The protein TON_0340 (268 amino acids) was identified in a transcriptome study aimed at identifying genes whose expression is enhanced when this organism was grown with CO as the sole carbon and energy source. The biological function of TON_0340 is unknown, and a BLAST database search shows that TON_0340 belongs to the DUF4392 superfamily (after domain of unknown function), the members of which are found in all three domains of life. To gain insights into the biochemical function of TON_0340 and its homologues, we determined the crystal structures of TON_0340 in four different forms; the apo form without a bound metal ion and the Mn2+-, Mg2+- or Ca2+-bound form, revealing that the protein has a highly conserved bi-metal binding pocket. Our analyses strongly support that TON_0340 is a novel Mn2+-dependent phosphatase.

The Ca2+-bound TON_0340 structure was determined by growing the crystals in the presence of CaCl2. Unexpectedly, only one Ca2+ ion bound to the cluster of the acidic residues. The Ca2+ ion was chelated by Glu59, Asp61, Glu115 and Asp157 occupying the Mn2 site. As anticipated, Ca2+ exhibited single-site interaction with TON_0340 with the deduced KD of 970 nM. Notably, TON_0340 was not activated by the addition of Ca2+ or Zn2+. Consistently, in the asymmetric unit of the Mn2+-, Mg2+-, Ca2+- or Zn2+-bound crystals, six molecules of TON_0340 formed three dimeric pairs which are essentially the same with each other, as if this observed homodimer is the biological unit. The two molecules in each pair are in antiparallel orientations. The intermolecular interactions, involving α1, α2 and α10, are mostly hydrophobic and quite extensive, burying a surface area of 1,202 Å2 in one subunit.

>[6x]MIAHLINTDIGNRGVLKVYLDYRRKNFNFLHNSTKMFLDNLERVLIVTGFPIPPMMVAETDGPPGALAIYRAVEMLGGKAEILTYSEVEKALEPFGVSLARTPEPEDYSLIISVETPGRAADGRYYSMSALEIKRDPLDGIFLKARALGIPTIGVGDGGNEIGMGKIRELVVGHVPHGEKIASVVETDELIVSAVSNWGAYGLVAQASIEVGRNLLEGWDERRVIEAISSAGLIDGVSKTLAPSVDGIRLMVHEGIVELLKAVVDEAIL>[6x]MEQSHQNLQSQFFIEHILQILPHRYPMLLVDRITELQANQKIVAYKNITFNEDVFNGHFPNKPIFPGVLIVEGMAQSGGFLAFT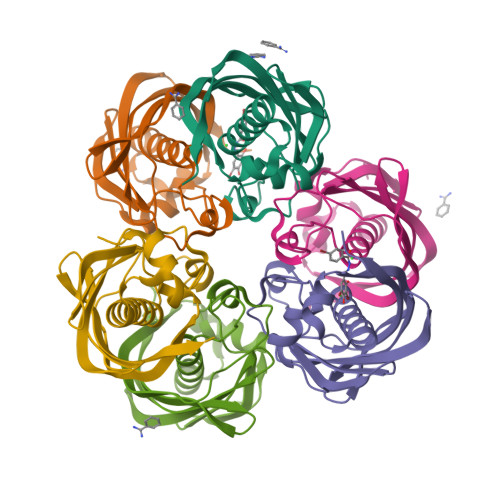SLWGFDPEIAKTKIVYFMTIDKVKFRIPVTPGDRLEYHLEVLKHKGMIWQVGGTAQVDGKVVAEAELKAMIAERE>[2x]AFKLPNLPYAYDALEPYFDQRTMEFHHDKHHNTYVTKLNATVEGTELEHQS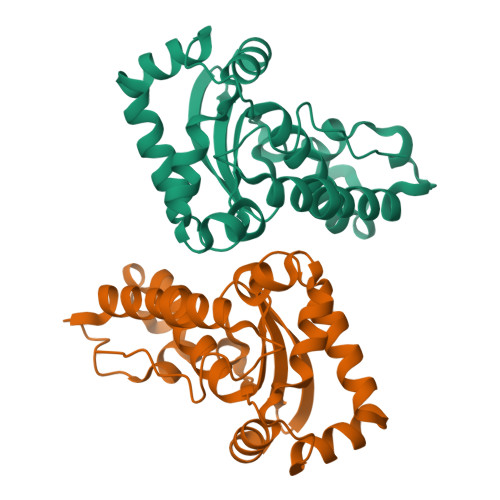LADMIANLDKVPEAMRMSVRNNGGGHFNHSLFWEILSPNSEEKGGVIDDIKAQWGTLDEFKNEFANKATTLFGSGWTWLVVNDGKLEIVTTPNQDNPLTEGKTPILGLDVWEHAYYLKYQNKRPDYMTAFWNIVNWKKVDELYQAAK> MGVIVELIDHTSAIAAAKDRADLVERLRAAKARISDPQIRVVIAGQLKQGKSQLLNSLLNIPVARVGDDESTVLATVVSYGEQASARLVVARPDGAEPELIEIPPSEVTTDLRRAPQASGRQVLRVEVTAPSPLLKGGLAFVDTPGVGGHGQPHLSATLGLLPDADAMLMISDTSQEFTEPEMKFIRQALEICPVAAI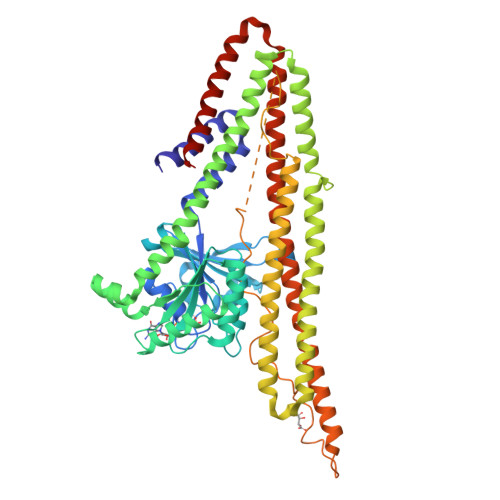VATKTDLYPHWRQIVDANIAHLQRAGLNVPVIPASSVLRSHAISLNDKELNEESNFPAIVKFLSEHVLSRQNDRIRDQIVDEIRSAAEHLLLAVESELSSFNDPGERERLTAELERRKQEAQDALQQTALWQQVLSDGIADLTADVDHDLRHRFRIIAAHTEKVIDGCDPTLHWAEIGAELEDAVATAVGDNFVWAYQRAEALAAEVARTFTEAGLDAVQMPQIDARDMGAGFGELNSLARLEAKPIKIGHKVVTGMRGSYGGVLMFGMLTSFAGLGMFNPLSLGAGFVLGRKAYKEDMENRMLRVRNEAKANVRKFVDDVAFVVGKESRDRLKGIQRQLRDHYREIANQTTRSLNESLQAAIAAAKVEEAERNTRVKELERQQNILKQVVDHAAKLAAALEHHHHHH> LKESPSGYLRSGEGDTGCGELVWVGEPLTLRTAETITGKYGVWMRDPKPTYPYTQETTWRIDTVGTDVRQVFEYDLISQFMQGYPSKVHILPRPLESTGAVVYSGSLYFQGAESRTVIRYELNTETVKAEKEIPGAGYHGQFPYSWGGYTDIDLAVDEAGLWVIYSTDEAKGAIVLSKLNPENLELEQTWETNIRKQSVANAFIICGTLYTVSSYTSADATINFAYDTGTGISKTLTIPFKNRYKYSSMIDYNPLEKKLFAWDNLNMVTYDIKLSKM

Inherited missense mutations in the myocilin (MYOC) gene, within its olfactomedin (OLF) domain, constitute the strongest genetic link to primary open-angle glaucoma via a toxic gain of function, and thus MYOC is an attractive precision-medicine target. Myocilin has no known function, and there is no glaucoma phenotype in Myoc knockout mice or in individuals with a homozygous N-terminal truncation mutation or hemizygous deletion of MYOC, but rare non-synonymous coding mutations lead to toxic intracellular sequestration of misfolded myocilin. However, not all mutations in MYOC cause glaucoma, and common variants are expected to be neutral polymorphisms. Among the common features associated with pathogenic myocilin misfolding, we demonstrate that a single metric, OLF thermal stability, can robustly segregate benign from early-onset disease variants.

V449I, a conservative substitution found in a hydrophobic region of the OLF β-propeller, appears only in gnomAD. Assessment of spent media from cells expressing each of the 16 full-length myocilin variants revealed WT-like secretion for T256M, R296H, L303I, S313F, V329M, S331L, T353I, A445V, V449I and K500R. Structural integrity was further confirmed by high-resolution crystal structures, which were solved for 11 OLF variants. No gross changes from WT OLF were detected for the structures of T293K, R296H, L303I, V329M, S331L, E352K, T353I, K398R, A445V, V449I or K500R, indicating that these mutations are accommodated within the native five-bladed β-propeller fold and do not perturb the dinuclear calcium-containing site.>GAMAVIDNSTKTLEQQTAQTNVAALPAITVKAEQDDTYAGGQVATSSNVGFLGSKKFLDTPFNTISYTDKYIEDKQAKDITEVIAATDPSIYTNGASGGWSENYYIRGYASSTNDMSMNGLFGITPFYRTSPEMFGRVEVLKGPSALLNGMPPAGSVGGTVNLVTKYAADEPFARLTTTYMSDAQFGGHVDVGRRFGENKEFGVRINGMYRDGDAAVNDQSKESRLFSLGLDWQGENARVFVDAYDALDHVDGVTRGVNVSTAVGIPKPPKADTLLSPDWGSVETKDKGAMIRGEYDFSDQLMAYAAYGQSTTEYKYNGASAGTITSSTGTLSSTLGQLAFDVDKKSADAGFKGKFETGSVKHQWVANATYYNHTQDDYSYRIIPGFSDPVIT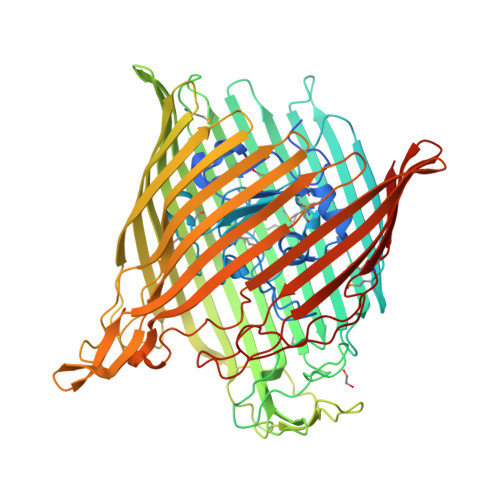NIYDPNPNWGPKPEFTPPFLFHSTLSTSSFGLADTLSFAQDKVQLTLGLRHQTVKATSSVNTLPENAKSATTPGVALLIKATDKISVYANYIEGLTKGDQAPATASNPGEIFPPQKTKQQELGLKVDLGTFAHTLSAFEITKPSSYLDPSKLVNNLPTFVSDGEQRNRGIEWSFFGSPIEHVRLMGGFTYLDPELTKTKSGGNDGHTAVAVPKNQAKLGAEWDTQVAQGTLTLSGNINAVSKQYINAENTLSVPGRTLLDVGARYSTKVEDHPVTFRANIYNLTNKAYWAQPQLTNLALGAPRTYMLSVSYDF[3x]> FQGMLPRDERRGQLLVVASDVFVDRGYHAAGMDEIADRAGVSKPVLYQHFSSKLELYLAVLHRHVENLVSGVHQALSTTTDNRQRLHVAVQAFFDFIEHDSQGYRLIFENDFVTEPEVAAQVRVATESCIDAVFALISADSGLDPHRARMIAVGLVGMSVDCARYWLDADKPISKSDAVEGTVQFAWG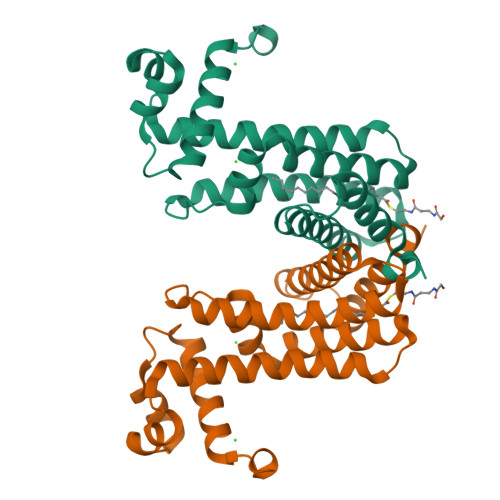GLSHVPL> HMRHKDCLLREFRKLCAMVADNPSYNTKTQIIQDFLRKGSAGDGFHGDVYLTVKLLLPGVIKTVYNLNDKQIVKLFSRIFNCNPDDMARDLEQGDVSETIRVFFEQSKSFPPAAKSLLTIQEVDEFLLRLS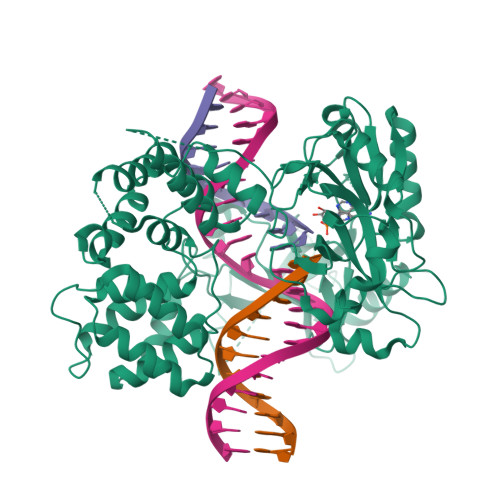KLTKEDEQQQALQDIASRCTANDLKCIIRLIKHDLKMNSGAKHVLDALDPNAYEAFKASRNLQDVVERVLHNAQEVEKEPGQRRALSVQASLMTPVQPMLAEACKSVEYAMKKCPNGMFSEIKYDGERVQVHKNGDHFSYFSRSLKPVLPHKVAHFKDYIPQAFPGGHSMILDSEVLLIDNKTGKPLPFGTLGVHKKAAFQDANVCLFVFDCIYFNDVSLMDRPLCERRKFLHDNMVEIPNRIMFSEMKRVTKALDLADMITRVIQEGLEGLVLKDVKGTYEPGKRHWLKVKKDYLNEGAMADTADLVVLGAFYGQGSKGGMMSIFLMGCYDPGSQKWCTVTKCAGGHDDATLARLQNELDMVKISKDPSKIPSWLKVNKIYYPDFIVPDPKKAAVWEITGAEFSKSEAHTADGISIRFPRCTRIRDDKDWKSATNLPQLKELYQLSK> ESCEYTCGSTCYWSSDVSAAKAKGYSLYESGDTIDDYPHEYHDYEGFDFPVSGTYYEYPIMSDYDVYTGGSPGADRVIFNGDDELAGVITHTGASG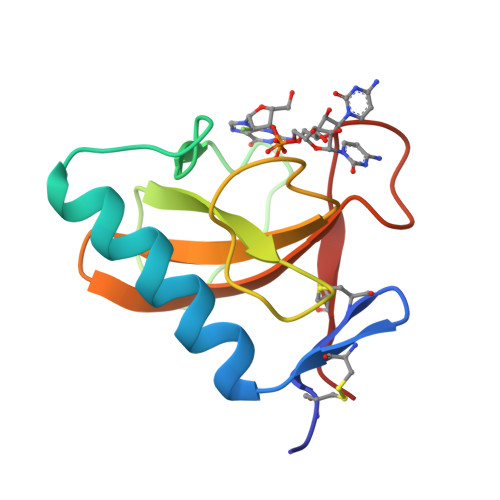DDFVACSSS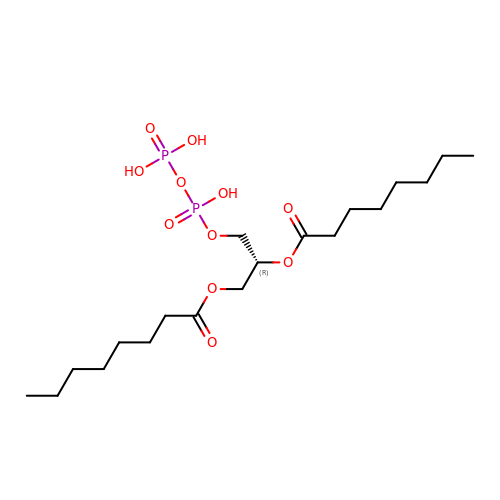(2R)-3-{[(R)-hydroxy(phosphonooxy)phosphoryl]oxy}propane-1,2-diyl dioctanoate | C19 H38 O11 P2 | MBDSUZSCJLRKPC-QGZVFWFLSA-N In this study, we explore M. abscessus phosphopantetheine adenylyl transferase (PPAT), an enzyme involved in the biosynthesis of Coenzyme A, as a target for the development of new antibiotics. Phosphopantetheine adenylyltransferase (PPAT or CoaD) catalyses the penultimate step in the biosynthesis of CoA in prokaryotes. The enzyme catalyses the reversible transfer of an adenylyl group from ATP to 4′-phosphopantetheine (PhP) to yield 3′-dephospho-CoA (dpCoA) and pyrophosphate. Further studies on M. tuberculosis show the essential role played by the coaD gene in mycobacterial growth in vitro, confirming the potential of PPAT as an antibiotic target.

Previous studies on E. coli PPAT have shown that Coenzyme A (CoA), the end-product of the biosynthetic pathway, acts as feedback inhibitor of the PPAT enzyme catalyzed reaction. To further understand the binding mode of CoA, we determined the crystal structure of Mab PPAT in complex with CoA. CoA and the enzyme product 3′-dephospho CoA (dpCoA) differ only by the presence of a 3-phosphate on the ribose ring. A structural superposition of the Mab PPAT CoA structure with that of dpCoA bound form determined, previously within our research group, shows that the pantetheine moiety of CoA and that of dpCoA adopts a similar conformation in the Mab PPAT active site. On the contrary, the adenosine moieties of CoA and dpCoA do not coincide in the Mab PPAT active site. The adenine ring along with the 3′-phosphate group of CoA is found largely exposed to the central solvent filled channel in Mab PPAT-CoA structure whereas in Mab PPAT-dpCoA, the adenine ring adopts a different position near the catalytic Arg90. Further, the adenyl moiety of CoA exhibits high B-factors in comparison to that of the dpCoA complex, suggesting greater movements of this moiety in CoA-bound Mab PPAT. This could be attributed to the steric hindrance in the molecule imparted by the additional phosphate group of CoA. Whereas in apo, PhP-bound and CoA-bound PPAT structures, the solvent channel adopts an open conformation and has a predominantly negative charge distribution from the acidic groups like Asp-94 and Glu-96 that are exposed to the channel.

>SMTGAVCPGSFDPVTLGHLDVFERAAAQFDEVIVAVLINPNKAGMFTVDERIEMIRESTADLPNLRVESGQGLLVDFVRERGLNAIVKGLRTGTDFEYELQMAQMNKHIAGVDTFFVATAPAYSFVSSSLAKEVATYGGDVSALLPASVHQRLLGKLRGQAQ[3x]The Phox homology (PX) domain was first identified in the NADPH phagocyte oxidase complex subunits p40phox and p47phox, and has since been found in proteins in every eukaryotic species from yeast to human. Despite relatively low overall sequence homology, PX domains all possess the same core fold, consisting of three antiparallel β-strands (β1-β3), followed by three α-helices (α1–α3). An extended sequence traverses the protein between helices α1 and α2, termed the PPK loop as it generally contains a conserved ΨPxxPxK motif (Ψ = large aliphatic amino acids V, I, L, and M). Side chains of residues from the β3 strand, α1 helix and PPK loop together form a binding pocket for the headgroup of the canonical lipid PtdIns3P.

We have also obtained two crystal structures of SGK3 and SNX23 (for which previous structures exist), as well as a crystal structure of SNX15, the crystal structure of SNX32 (in complex with a peptide from the bacterial IncE peptide) and the NMR structure of SNX25. Last, we observe an unusual domain-swapped structure and membrane-binding activity of the SNX15 PX domain. Interestingly, our binding data are similar to that shown previously for the isolated SNX15 PX domain; in contrast, however, the full-length SNX15 protein bound relatively strongly to PtdIns3P24. Further work will be needed to clarify the functional oligomeric state and membrane binding of this protein.

> GSMSRQAKDDFLRHYTVSDPRTHPKGYTEYKVTAQFISKKDPEDVKEVVVWKRYSDFRKLHGDLAYTHRNLFRRLEEFPAFPRAQVFGRFEASVIEERRKGAEDLLRFTVHIPALNNSPQLKEFFRGG> MEEQD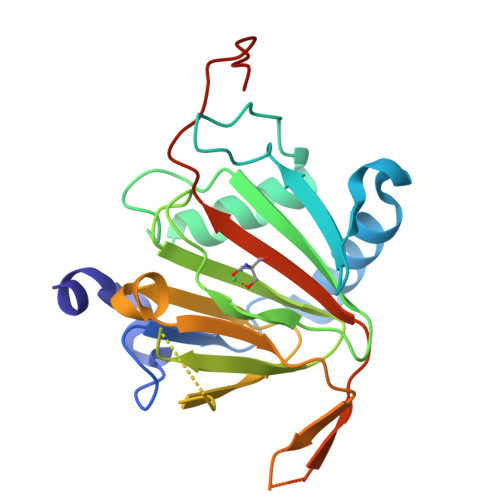ARVPALEPFRVEQAPPVIYYVPDFISKEEEEYLLRQVFNAPKPKWTQLSGRKLQNWGGLPHPRGMVPERLPPWLQRYVDKVSNLSLFGGLPANHVLVNQYLPGEGIMPHEDGPLYYPTVSTISLGSHTVLDFYEPRRPEDDDPTEQPRPPPRPTTSLLLEPRSLLVLRGPAYTRLLHGIAAARVDALDAASSPPNAAACPSARPGACLVRGTRVSLTIRRVPRVLRAGLLLGKGTENLYFQ> SEDCENIFHDNAYLLKLDCEAGRVDPVEYDDISDEEIYEITVDVGVSSEDQEKVAKIIRECIAQVSTQDCT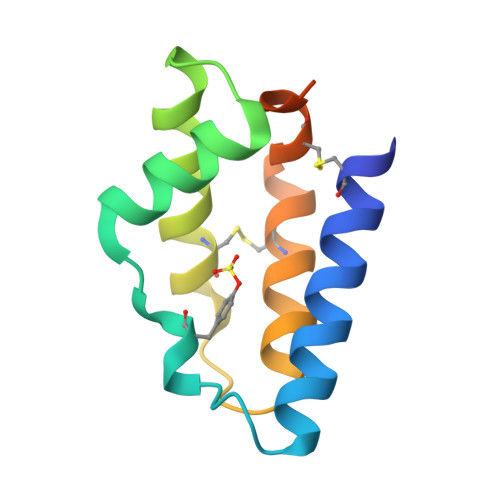KFSEIYDCYMKKKICNYYPENMGSGHHHHHHHH>QKEQHSQLNQTKIAYEQRLLNDLEDMDDPLDLFLDYMIWISTSYIEVDSESGQEVLRSTMERCLIYIQDMETYRNDPRFLKIWIWYINLFLSNNFHESENTFKYMFNKGIGTKLSLFYEEFSKLLENAQFFLEAKVLLELGAENNCRPYNRLLRSLSNYEDRLREMNIVENQNSVPDSRERLKGRLIYRTAPFF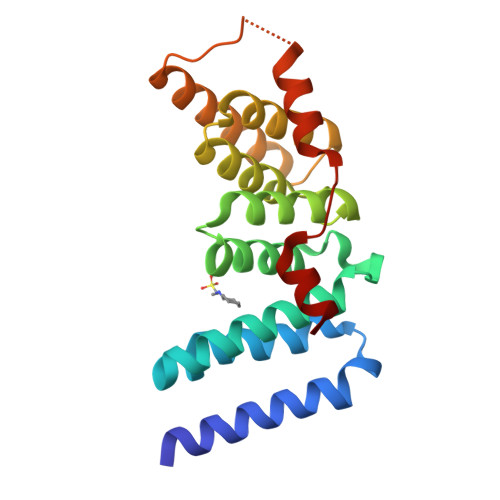IRKFLTSS[2x]>[24x]MTEYEGPKTKFHALMQEQIHNEFTAAQ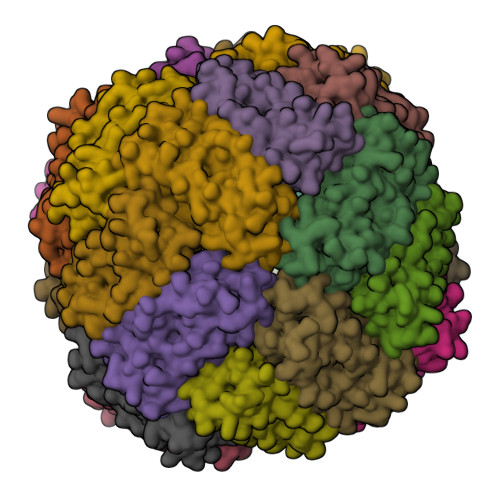QYVAIAVYFDSEDLPQLAKHFYSQAVEERNHAMMLVQHLLDRDLRVEIPGVDTVRNQFDRPREALALALDQERTVTDQVGRLTAVARDEGDFLGEQFMQWFLQEQIEEVALMATLVRVADRAGANLFELENFVAREVDVAPAASGAPHAAGGRLGSHHHHHH> MSKEIPTPYMWSYQPQMGLAAGAAQDYSTRINYMSAGPHMISRVNGIRAHRNRILLEQAAITTTPRNNLNPRSWPAALVYQESPAPTTVVLP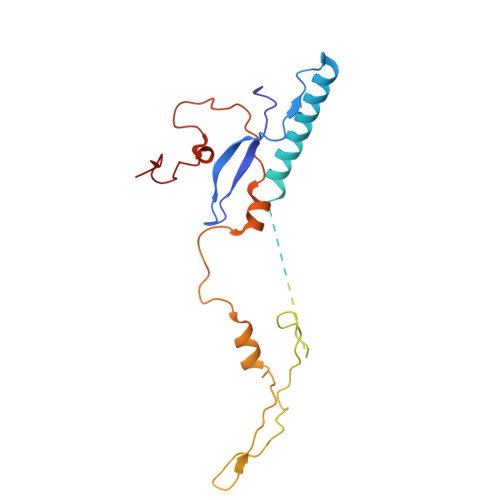RDAQAEVQMTNSGAQLAGGFRHRVRSPGQGITHLTIRGRGIQLNDESVSSSLGLRPDGTFQIGGAGRPSFTPRQAILTLQTSSSEPRSGGIGTLQFIEEFVPSVYFNPFSGPPGHYPDQFIPNFDAVKDSADGYD>[2x]METIAVHAGPRPYEDQAVLGAIRAAIKGLQALSFRYEGGSTPGRTREVTPLGVLFGRSNYLVALEGKGGKPRSWRLDRMSDLKVLDKPAPPPQDFSLQAFADESFGIYHDEI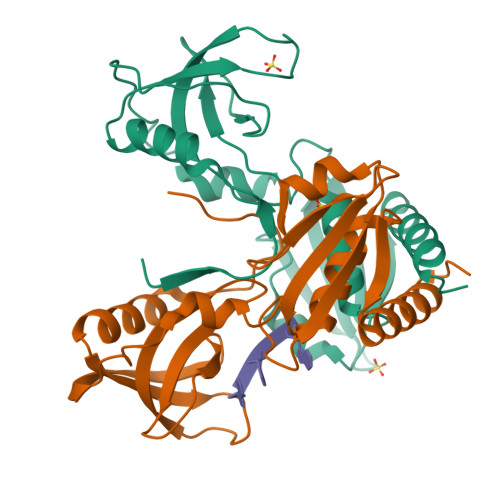QDVVLRIHKSRAEDALRWRFHATQQVTPEADGSVLVTFRAGGMRELSWHLFTWGDAVEIVAPQVLKDMMVQELREAGRAHGAW>[2x]GMVPMTRFDSATEVVRVGENRYAVELDPGYLIGTAMNGGYLMTVLQRSALAESDHLHAVSSS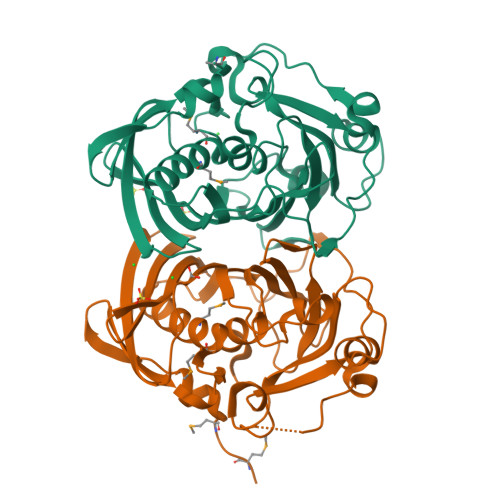YHFHRPASSGPAEIETRVLKRGRTVTTVQTTLFQEGRTILTGTLATATLDPHAEPRYAAPQPAIPPQHQCRRVDPRQSHLPDDGFLARVDVDFSPDSYAALARERTVTTPELCGYVDLSARDGGSAKDPLAFLPLAVDALPPIVSLLVDWSWAPTVELTWHLRAIPEPGPLAFRSTCALVSDGWFDENVDLWDARGRLVAQSRQLARVGR HP activity is regulated by its first and rate-limiting enzyme glutamine fructose-6-phosphate amidotransferase (GFAT, EC 2.6.1.16). GFAT is a modular enzyme composed of a glutaminase domain responsible for hydrolysis of l-Gln into l-glutamate (l-Glu) and an isomerase/transferase domain that catalyzes the isomerization of Frc6P to glucose-6-phosphate (Glc6P) as well as the transfer of ammonia to Glc6P to build glucosamine-6-phosphate (GlcN6P). The relative orientation of the two domains with their respective active sites is relevant for catalysis and affected by substrate binding. GFAT-1 activity is modulated by UDP-GlcNAc feedback inhibition and via phosphorylation by protein kinase A (PKA).

Subsequently, we crystallized human GFAT-1 R203H to further elucidate the structural basis of the reduced UDP-GlcNAc sensitivity. The GFAT-1 R203H crystals diffracted to a resolution limit of 2.77 Å. Compared to wild type GFAT-1, the R203H substitution does not cause major structural changes. While Arg203 interacts with the backbone residues of Ile178 and Leu181, as well as with Asp279 in wild type GFAT-1, these interactions are abolished in the R203H GFAT-1. In the mutant enzyme, however, the side chain of His203 protrudes between Asp278 and Asp279, without affecting the orientation of the neighboring loop (residues 277–280). In contrast, UDP-GlcNAc dose response assays revealed an ~6-fold higher IC50 value of R203H GFAT-1 compared to wild type GFAT-1 (R203H: 231.7 −15.2/+16.3 µM; wild type: 41.4 −3.5/+3.9 µM). In addition to the observed gain-of-function caused by reduced feedback inhibition, the R203H substitution alters the PKA consensus sequence of Ser205 from RRGS to RHGS, suggesting a potential change of Ser205 phosphorylation and a subsequent loss of regulation. Thus, disruption of the PKA consensus sequence by the R203H substitution prevents PKA-mediated phosphorylation at Ser205. Here we present the GFAT-1 R203H gain-of-function variant and decipher the two consequences of the substitution: first, GFAT-1 R203H displays strongly reduced PKA-dependent phosphorylation at Ser205 due to a disrupted consensus sequence and, second, shows weaker sensitivity to UDP-GlcNAc feedback inhibition.

>MCGIFAYLNYHVPRTRREILETLIKGLQRLEYRGYDSAGVGFDGGNDKDWEANACKIQLIKKKGKVKALDEEVHKQQDMDLDIEFDVHLGIAHTRWATHGEPSPVNSHPQRSDKNNEFIVIHNGIITNYKDLKKFLESKGYDFESETDTETIAKLVKYMYDNRESQDTSFTTLVERVIQQLEGAFALVFKSVHFPGQAVGTRHGSPLLIGVRSEHKLSTDHIPILYRTGKDKKGSCNLSRVDSTTCLFPVEEKAVEYYFASDASAVIEHTNRVIFLEDDDVAAVVDGRLSIHRIKRTAGHHHHHHDHPGRAVQTLQMELQQIMKGNFSSFMQKEIFEQPESVVNTMRGRVNFDDYTVNLGGLKDHIKEIQRCRRLILIACGTSYHAGVATRQVLEELTELPVMVELASDFLDRNTPVFRDDVCFFLSQSGETADTLMGLRYCKERGALTVGITNTVGSSISRETDCGVHINAGPEIGVASTKAYTSQFVSLVMFALMMCDDRISMQERRKEIMLGLKRLPDLIKEVLSMDDEIQKLATELYHQKSVLIMGRGYHYATCLEGALKIKEITYMHSEGILAGELKHGPLALVDKLMPVIMIIMRDHTYAKCQNALQQVVARQGRPVVICDKEDTETIKNTKRTIKVPHSVDCLQGILSVIPLQLLAFHLAVLRGYDVDFPRNLAKSVTVE[2x]TRIM E3 ubiquitin ligases regulate a wide variety of cellular processes and are particularly important during innate immune signalling events. They are characterized by a conserved tripartite motif in their N‐terminal portion which comprises a canonical RING domain, one or two B‐box domains and a coiled‐coil region that mediates ligase dimerization. The RING domain of TRIMs adopts the canonical RING domain fold that recognizes the ubiquitin‐loaded E2 conjugating enzyme (E2~Ub). To understand the role of self‐association and gain insight into the mechanism of TRIM‐mediated ubiquitination, we have analysed the properties of two TRIM ligases, TRIM25 and TRIM32, which differ in their domain architecture with TRIM25 containing two B‐boxes compared to a single B‐box2 in TRIM32.

In contrast, a fragment that is extended by 10 and 9 residues N‐ and C‐terminally, which are predicted to be α‐helical, is dimeric at all concentrations tested, suggesting that TRIM32 might dimerize in a manner similar to that of a number of homo‐ and heterodimeric RING ligases such as the BRCA1/BARD1 complex, where N‐ and C‐terminally located α‐helices form a four‐helix bundle (Brzovic et al, 2001). The extended RING domain of TRIM32 crystallized as a dimer with a significant proportion of the dimer interface formed by two α‐helices located N‐ and C‐terminal to the core RING domain, respectively, that form a four‐helix bundle. Dimerization buries 970 A2 and the dimer interface is formed predominantly by hydrophobic residues located within the four helices. RING dimerization through a four‐helix bundle employing regions outside the RING has been observed in a number of dimeric RINGs such as the BRCA1/BARD1 heterodimer or the Rad18 homodimer (Brzovic et al, 2001; Huang et al, 2011). The RINGs of TRIM32 are constitutive dimers even in the absence of the rest of the remainder of the protein or additional binding partners. In contrast, we could not detect activity for the monomeric TRIM32 core RING domain. However, the extended dimeric RING showed a similar level of activity as the B‐box‐containing fragment, which was further enhanced in the tetrameric TRIM32 RBCC construct albeit to a much lower extend compared to TRIM25. In support of a more general role of this acidic residue, mutation of the equivalent E16 in TRIM32 also disrupts catalytic activity. This effect is similar to the mutation of I85R, which interferes with dimerization, similar to V72R in TRIM25 (and EV2).

>[2x]MSHLNLDALREVLECPICMESFTEEQLRPKLLHCGHTICRQCLEKLLASSINGVRCPFCSKITRITSLTQLTDNLTVLKIIDTAGLSEHHHHHH ethyl 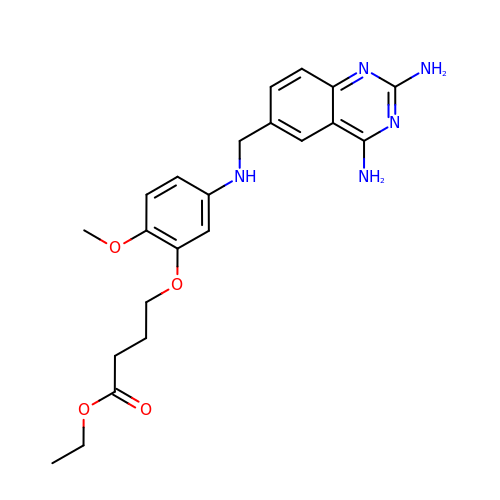4-(5-{[(2,4-diaminoquinazolin-6-yl)methyl]amino}-2-methoxyphenoxy)butanoate | C22 H27 N5 O4 | YUHXPHNBJFUHSN-UHFFFAOYSA-N octyl beta-L-talopyranoside | C14 H28 O6 | 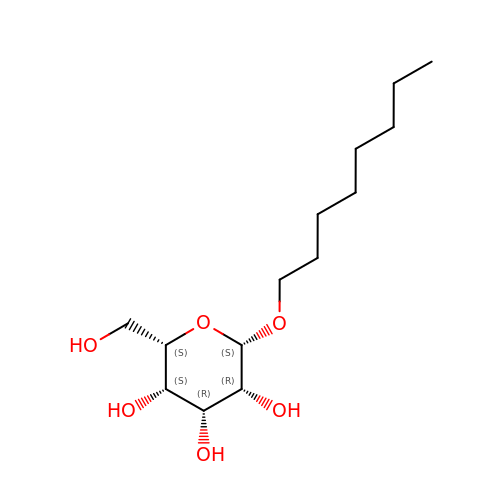HEGSGKPQLMEBJL-MRTXSQPYSA-N> IVGGYTCGANTVPYQVSLNSGYHFCGGSLINSQWVVSAAHCYKSGIQVRLGEDNINVVEGNEQFISASKSIVHPSYNSETYNNDIMLIKLKSAASLNSRVASISLPTSCASAGTQCLISGWGNTKSSGTSYPDVLKCLKAPILSDSSCKSASSFIITSNMFCAGYLEGGKDACQGDSGGPVVCSGKLQGIVSWGEGC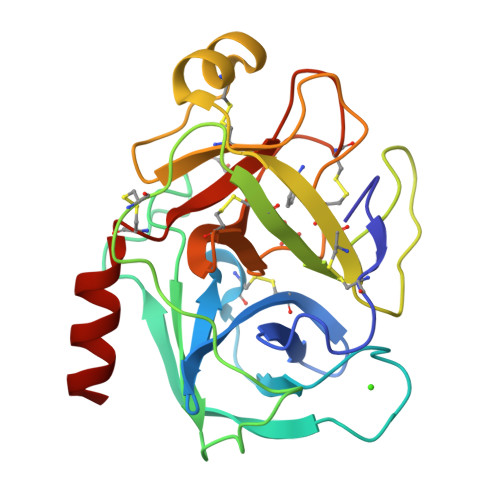AQKNKPGIYTKVCNYVSWIKQTIASN> PVW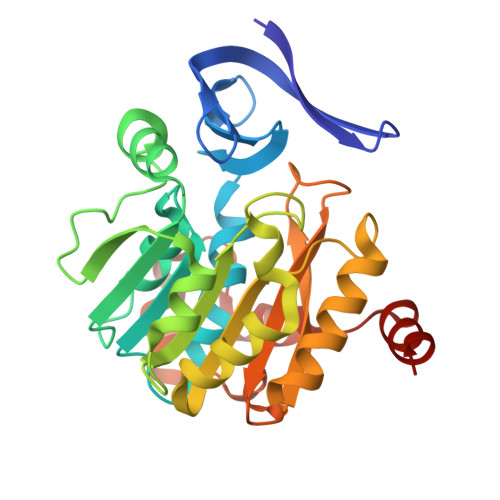IDEVFEDRVRYGLRGQILWEETSPFQKITIVDTEHYGRGLLLDDCWMTAERCEVCYHEYLVHPPLTTAASIARVLVIGGGDGGTVREVLRYAEVEQVDLVEIDGRVVELSQEYLGAIGTAWADPRLNVKIGDGIAFVQTAPDASYDVILVDGSDPAGPAAGLFNREFYENCRRVLKPGGVFASQAESPDSFLAVHLEMIETLSAVFAEAKPYYGWVPMYPSGWWSWLYASDTPGQFQKPQSDRLAAIEPQVEIYNRDIHQAAFAQPNFVRRGLSARQ>ADPWQECMDYAVTLARQAGEVVCEAIKNEMNVMLKSSPVDLVTATDQKVEKMLISSIKEKYPSHSFIGEESVAAGEKSILTDNPTWIIDPIDGTTNFVHRFPFVAVSIGFAVNKKIEFGVVYSCVEGKMYTARKGKGAFCNGQK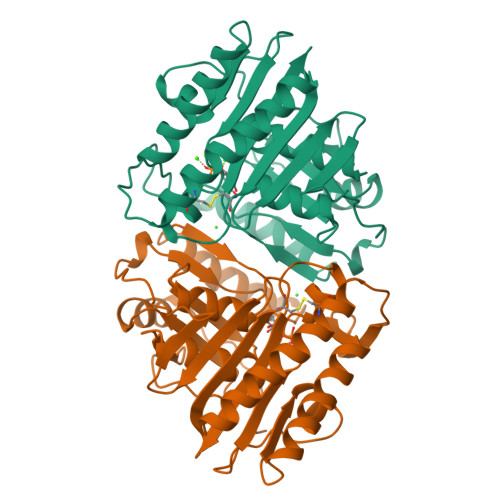LQVSQQEDITKSLLVTELGSSRTPETVRMVLSNMEKLFCIPVHGIRSVGTAAVNMCLVATGGADAYYEMGIHCWDVAGAGIIVTEAGGVLMDVTGGPFDLMSRRVIAANNRILAERIAKEIQVIPLQRDDED[2x]4,4,4-tris(fluoranyl)-~{N}-isoquinolin-6-yl-butane-1-sulfonamide | C13 H13 F3 N2 O2 S | 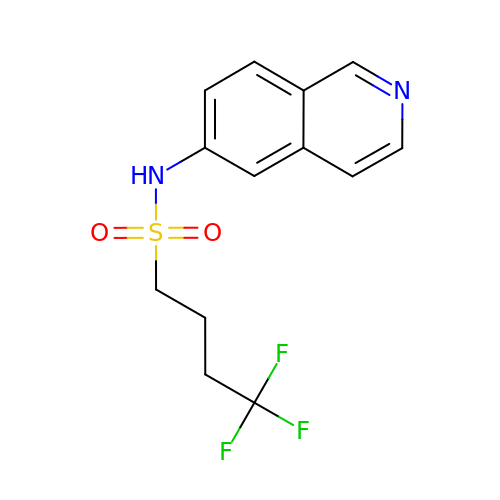MPUJMWAAXOTDHM-UHFFFAOYSA-N>AEAGITGTWYNQLGSTFIVTAGADGALTGTYESAVGNAESRYVLTGRYDSAPATDGSGTALGWTVA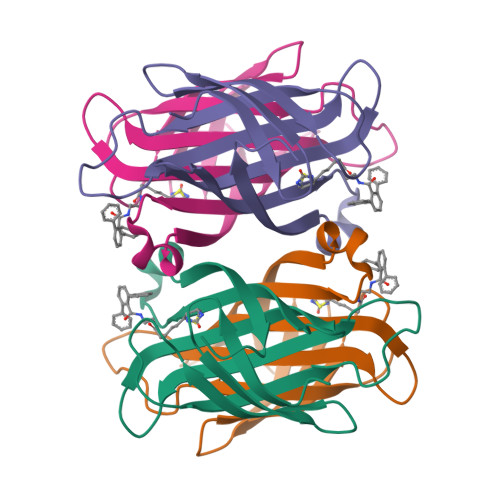WKNNYRNAHSATTWSGQYVGGAEARINTQWLLTSGTTEANAWKSTLVGHDTFTKVKPSAAS[2x]>MSVSSLLEVVADDLLKLNNNLKSLVGAENPVLVSAAEQIFGAGGKRLRPALVFLVSRATAELAGLLELTTEHQRLAEIIEMIHTASLIHDDVIDDSGMRRGKETIHQLYGTRVAVLAGDFMFAQSSWFLANLENIEVIKLISQVIKDFASGEIKQASTLFDCDITLDDYLLKSYYKTASLIAASTRSAAIFSGVSTAICEQMYEYGRNLGLSFQVVDDILDFTQSAEQLGKPAGSDLAKGNLTAPVIFALQDEPQLREIIDSEFSETNSLATAIELVHRSGGIKRAHELAREKGEIAIQSLQCLPRSEFRSTLENMVKYNLERID[2x];>EAALGDAKDALYAALEGMNRGIFGMTSEKRSEIHALVELLESKNPTPEPTDKLQDKVDGCWRLVYSTISILGKKRTKLGLRDFISLGDFFQMIDVKEEKAVNVIKFSARALKILSGQLTIEASYKITTKTKVDITLDSST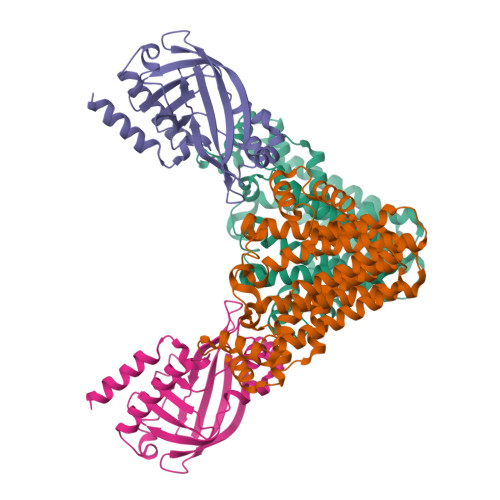ITPDQLMNIFQKNYDMLLAIFNPEGWLEITYVDESLRIGRDDKANIFVLERADPSEV[2x]> VVGGTEAQRNS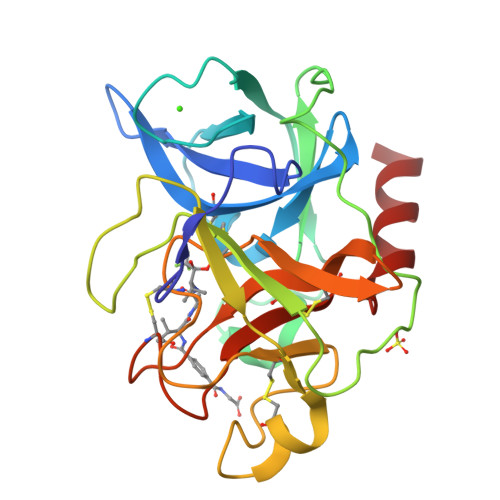WPSQISLQYRSGSSWAHTCGGTLIRQNWVMTAAHCVDRELTFRVVVGEHNLNQNDGTEQYVGVQKIVVHPYWNTDDVAAGYDIALLRLAQSVTLNSYVQLGVLPRAGTILANNSPCYITGWGLTRTNGQLAQTLQQAYLPTVDYAICSSSSYWGSTVKNSMVCAGGDGVRSGCQGDSGGPLHCLVNGQYAVHGVTSFVSRLGCNVTRKPTVFTRVSAYISWINNVIASN> MTGPILSGLDPRFERTLYAHVGKEGSWTLDYYLRHGGYETAKRVLKEKTPDEVIEEVKRSGLRGRGGAGFPTGLKWSFMPKDDGKQHYLICNADESEPGSFKDRYILEDVPHLLIEGMILAGYAIRATVGYIYVRGEYRRAADRLEQAIKEARARGYLGKNLF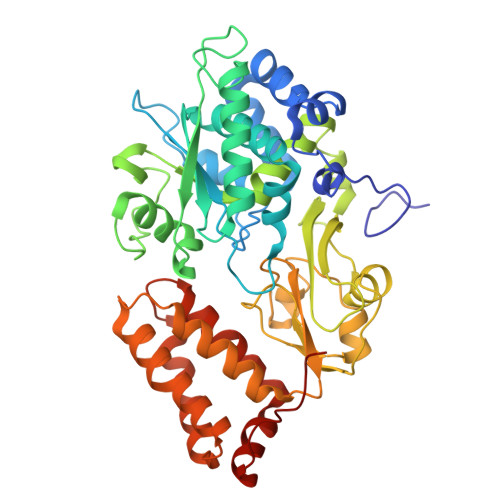GTDFSFDLHVHRGAGAYICGEETALMNSLEGLRANPRLKPPFPAQSGLWGKPTTINNVETLASVVPIMERGADWFAQMGTEQSKGMKLYQISGPVKRPGVYELPMGTTFRELIYEWAGGPLEPIQAIIPGGSSTPPLPFTEEVLDTPMSYEHLQAKGSMLGTGGVILIPERVSMVDAMWNLTRFYAHESCGKCTPCREGVAGFMVNLFAKIGTGQGEEKDVENLEALLPLIEGRSFCPLADAAVWPVKGSLRHFKDQYLALAREKRPVPRPSLWR>[2x]MPYRNCWSKIMKKLINDVQDVLD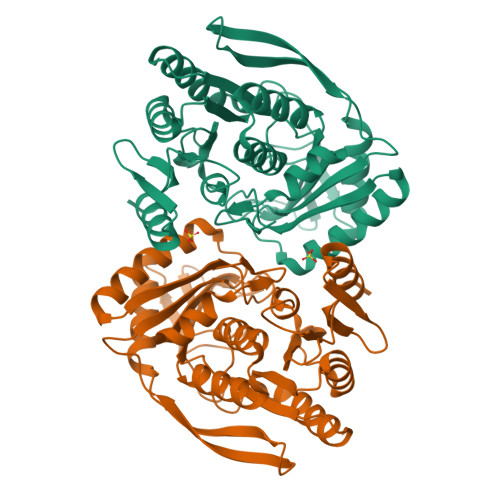EQLAGLAKAHPSLTLHQDPVYVTRADAPVAGKVALLSGGGSGHEPMHCGYIGQGMLSGACPGEIFTSPTPDKIFECAMQVDGGEGVLLIIKNYTGDILNFETATELLHDSGVKVTTVVIDDDVAVKDSLYTAGRRGVANTVLIEKLVGAAAERGDSLDACAELGRKLNNQGHSIGIALGACTVPAAGKPSFTLADNEMEFGVGIHGEPGIDRRPFSSLDQTVDEMFDTLLVNGSYHRTLRFWDYQQGSWQEEQQTKQPLQSGDRVIALVNNLGATPLSELYGVYNRLTTRCQQAGLTIERNLIGAYCTSLDMTGFSITLLKVDDETLALWDAPVHTPALNWGK> ISEFDYKDHDIDYKDDDDKWIMSLSIKELYYTKDKSINNVNLADGNY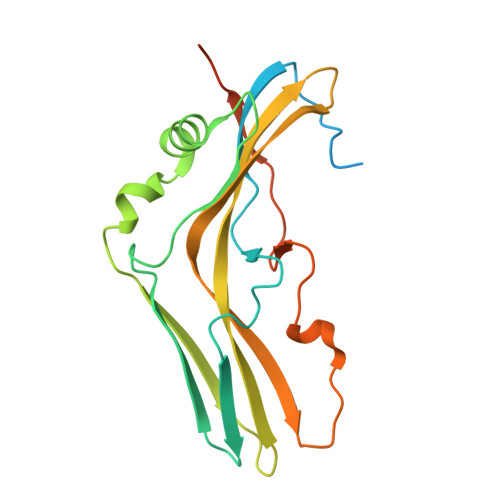VVNRGDGWILSRQNQNLGGNISNNGCTAIVGDLRIRETATPYYYPTASFNEEYIKNNVQNVFANFTEASEIPIGFEFSKTAPSNKSLYMYLQYTYIRYEIIKVLQNTVTERAVLYVPSLGYVKSIEFNSEEQIDKNFYFTSQDKCILNEKFIYKKIDDTITVKESKNSNNNINFNTS>[2x]GHMITHFRQAIEETLPWLSSFGADPAGGMTRLLYSPEWLETQQQFKKRMAASGLETRFDEVGNLYGRLNGTEYPQEVVLSGSHIDTVVNGGNLDGQFGALAAWLAIDWLKTQYGAPLRTVEVVAMAEAEGSRFPYVFWGSKNIFGLANPDDVRNICDAKGNSFVDAMKACGFTLPNAPLTPRQDI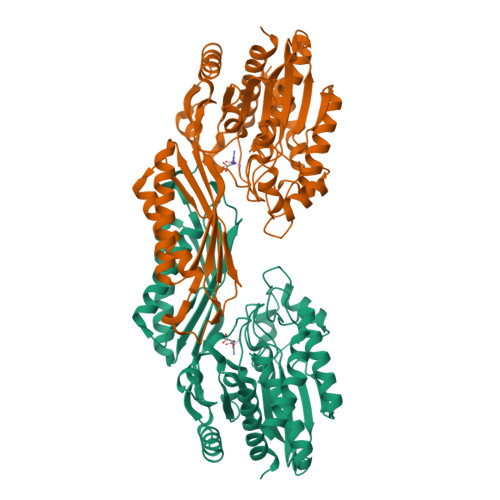KAFVELHIEQGCVLESNGQSIGVVNAIVGQRRYTVTLNGESNHAGTTPMGYRRDTVYAFSRICHQSVEKAKRMGDPLVLTFGKVEPRPNTVNVVPGKTTFTIDCRHTDAAVLRDFTQQLENDMRAICDEMDIGIDIDLWMDEEPVPMNKELVATLTELCEREKLNYRVMHSGAGHDAQIFAPRVPTCMIFIPSINGISHNPAERTNITDLAEGVKTLALMLYQLAWQK> GLPGMLTPDLAARLRLAFDDDRDAETFRLRLERYGPELADNLRAVYGNHADALIGELLEVMLHAYHARPADLKRLDEARLLRPDWLQGPEMVGYVAYVDRFAGTLRGVGERLEYLEGLGVTYLHLLPLLRPRDGENDGGYAVQDYRSVRPDLGTIDDLSALARELRGRGISLVLDLVLNHVAEEHEWAVRATAGEAAYRDYFHIFPDRTQPDAYERTLPEIFPDFAPGNFTWNGEAGGWVWTTFNRSQWDVNWGNPAVFREYLDLILTLANRGVEVFRLDAIAFLWKR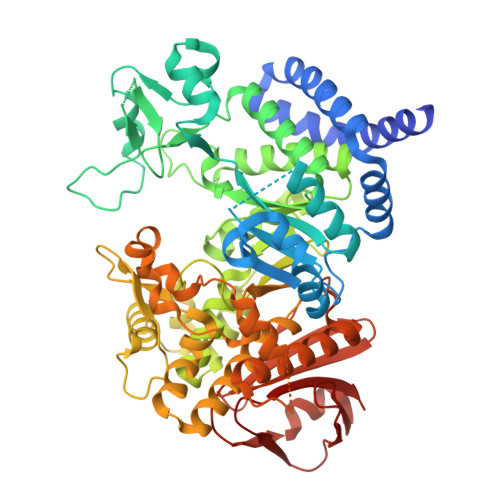LGTDCQNQPEVHRLTHALRAATRIVAPAVAFKAEAIVAPGDLIHYLGSRDHHGRVSDMAYHNSLMVQLWSSLASRDTRLLTAALAAFPPKPTNTTWGVYVRCHDDIGWAIADEDAARVGLSGPAHRHFLSDFYSGEFPGSFARGLVFQHHPQTGDRRISGTAASLAGLDLALETGDAERVNDALARLLLLHAVMLGFGGVPLLYMGDELALLNDTDFAAVPAHAADNRWVHRPQMDWELVASAQADAATGQPVTPAGRMFAGLRHLLAVRRRTPHLHASTESRPLPSPDPCVLLLRREHPTGVLLQVYNFSEHHITFPTWPLQEQLGAVAHDLLGESQFHLGGPDLALEPYRALWLVAGG>[2x]MNTTPVHALTDIDGGIAVDPAPRLAGPPVFGGPGNDAFDLAPVRSTGREMLRFDFPGVSIGAAHYEEGPTGATVIHIPAGARTAVDARGGAVGLSGGYDFNHAICLAGGAGYGLEAGAGVSRALLERLEHRTGFAELQLVSSAVIYDFSARSTAVYPDKALGRAALEFAVPGEFPQGRAGAGMSASAGKVDWDRTEITGQGAAFRRLGDVRILAVVVPNPVGVIVDRAGTVVR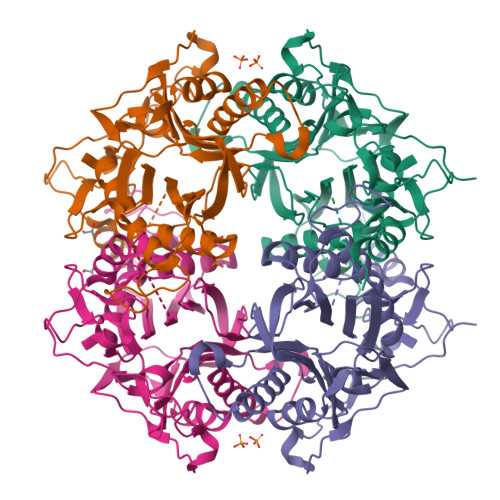GNYDAQTGVRRHPVFDYQEAFAEQVPPVTEAGNTTISAIVTNVRMSPVELNQFAKQVHSSMHRGIQPFHTDMDGDTLFAVTTDEIDLPTTPGSSRGRLSVNATALGAIASEVMWDAVLEAGK N-[(2H-1,3-benzodioxol-5-yl)methyl]-2-({[(2H-1,3-benzodioxol-5-yl)methyl][2-(chloromethyl)-1,3-oxazole-4-carbonyl]amino}methyl)-N-[(4-carbamoyl-1,3-oxazol-2-yl)methyl]-1,3-oxazole-4-carboxamide | C31 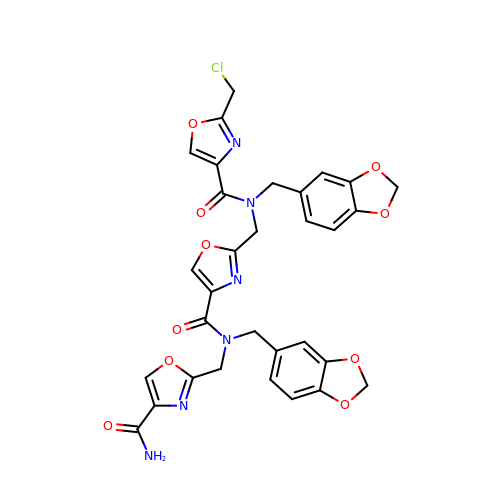H25 Cl N6 O10 | ZSCMZNFJKJBCQT-UHFFFAOYSA-N> GSHMAARRGALIVLEGVDRAGKSTQSRKLVEALCAAGHRAELLRFPERSTEIGKLLSSYLQKKSDVEDHSVHLLFSANRWEQVPLIKEKLSQGVTLVVDRYAFSGVAYTGAKENFSLDWCKQPDVGLPKPDLVLFLQLQLADAAKRGAFGHERYENGAFQERALRCFHQL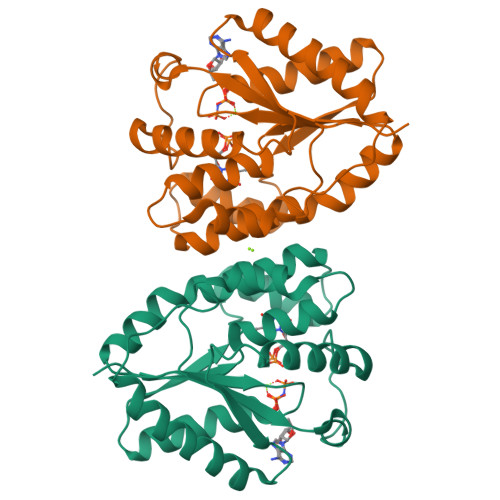MKDTTLNWKMVDASKSIEAVHEDIRVLSEDAIATATEKPLKELWK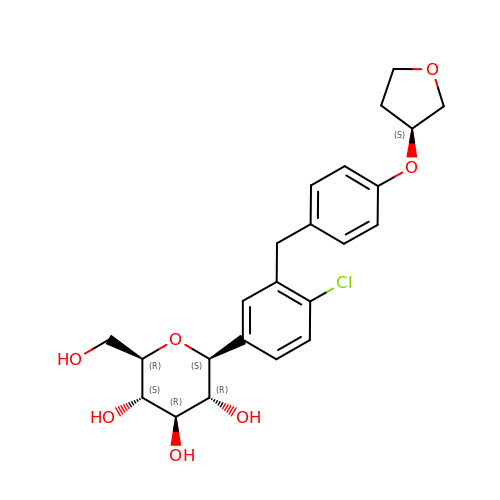(2S,3R,4R,5S,6R)-2-[4-chloranyl-3-[[4-[(3S)-oxolan-3-yl]oxyphenyl]methyl]phenyl]-6-(hydroxymethyl)oxane-3,4,5-triol | C23 H27 Cl O7 | OBWASQILIWPZMG-QZMOQZSNSA-N>[12x]MAPSRLCVYCADVCPDRLRCAAWLLATGIFLLLAGCSEAKAPTALERVQKEGVLRVITRNSPATYFQDRNGETGFEYELAKRFAERLGVELKIETADNLDDLYAQLSREGGPALAAAGLTPGREDDASV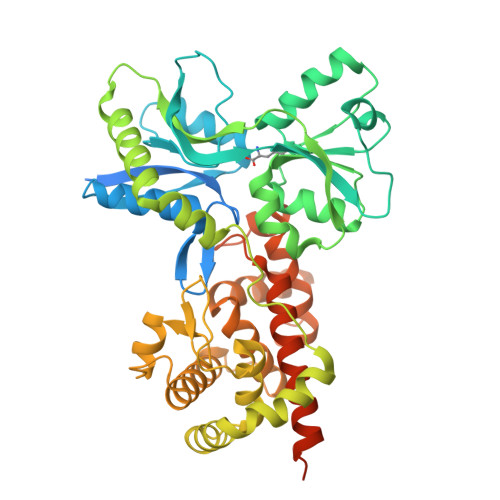RYSHTYLDVTPQIIYRNGQQRPTRPEDLVGKRIMVLKGSSHAEQLAELKKQYPELKYEESDAVEVVDLLRMVDVGDIDLTLVDSNELAMNQVYFPNVRVAFDFGEARGLAWALPGGDDDSLMNEVNAFLDQAKKEGLLQRLKDRYYGHVDVLGYVGAYTFAQHLQQRLPRYESHFKQSGKQKDTDWRLLAAIGYQESLWQPGATSKTGVRGLMMLTNRTAQAMGVSNRLDPKQSIQGGSKYFVQIRSELPESIKEPDRSWFALAAYNIGGAHLEDARKMAEKEGLNPNKWLDVKKMLPRLAQKQWYAKTRYGYARGGETVHFVQNVRRYYDILTWVTQPQMEGSQIAESGLHLPGVNKTRPEEDSGDEKL> DKMDYDFKVKLSSERERVEDLFEYEGCKVGRGTYGHVYKAKRKDGKDDKDYALKQIEGTGISMSACREIALLRELKHPNVISL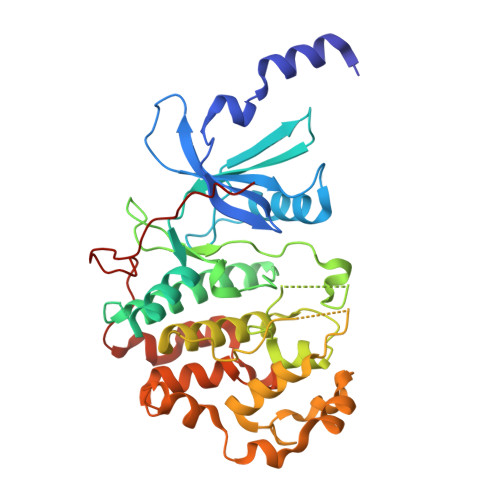QKVFLSHADRKVWLLFDYAEHDLWHIIKFHRASKANKKPVQLPRGMVKSLLYQILDGIHYLHANWVLHRDLKPANILVMGEGPERGRVKIADMGFARLFNSPLKPLADLDPVVVTFWYRAPELLLGARHYTKAIDIWAIGCIFAELLTSEPIFHCRQEDIKTSNPYHHDQLDRIFNVMGFPADKDWEDIKKMPEHSTLMKDFRRNTYTNCSLIKYMEKHKVKPDSKAFHLLQKLLTMDPIKRITSEQAMQDPYFLEDPLPTSDVFAGCQIPYPKREFLTEE1-(3-imidazol-1-ylpropyl)-5-(2-methylpropyl)-4-phenyl-imidazole | C19 H24 N4 | 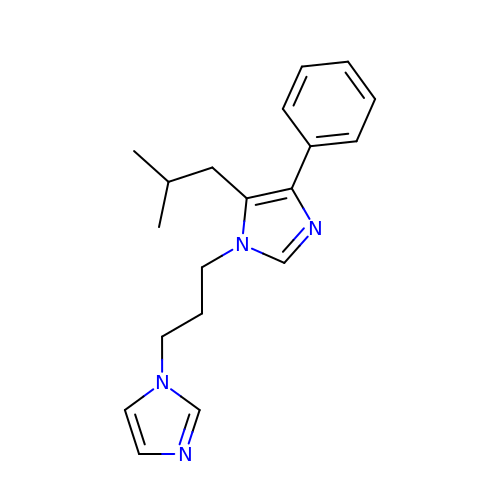WJQVYWBLSJRHQE-UHFFFAOYSA-N> MTQFAFVFPGQGSQTVGMLADMAASYPIVEETFAEASAALGYDLWALTQQGPAEELNKTWQTQPALLTASVALYRVWQQQGGKAPAMMAGHSLGEYSALVCAGVIDFADAVRLVEMRGKFMQEAVPEGTGAMAAIIGLDDASIAKACEEAAEGQVVSPVNFNSPGQVVIAGHKEAVERA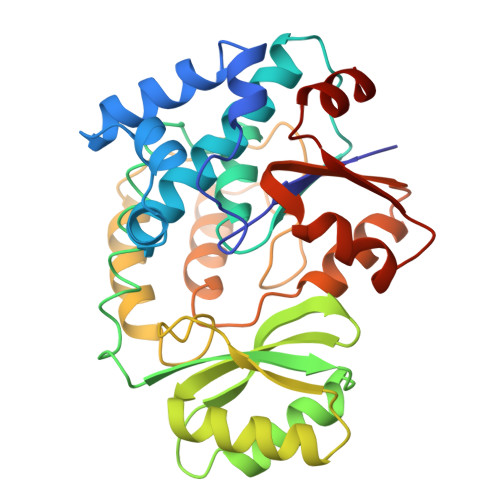GAACKAAGAKRALPLPVSVPSHCALMKPAADKLAVELAKITFNAPTVPVVNNVDVKCETNGDAIRDALVRQLYNPVQWTKSVEYMAAQGVEHLYEVGPGKVLTGLTKRIVDTLTASALNEPSAMAAALEL(2R)-2-(3-{[AMINO(IMINO)METHYL]AMINO}PHENYL)-3-SULFANYLPROPANOIC ACID | C10 H13 N3 O2 S | 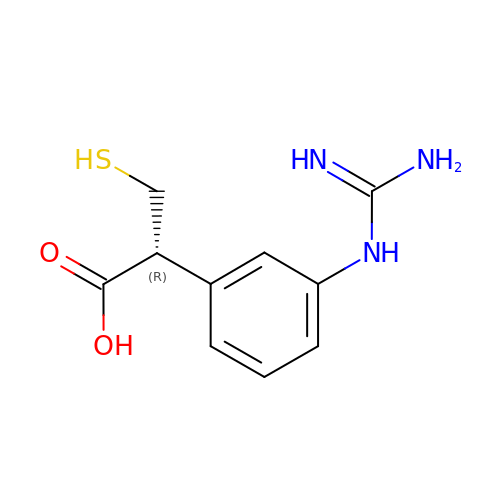YHBCRXAIIVZWEW-MRVPVSSYSA-N2-{5-[AMINO(IMINIO)METHYL]-1H-BENZIMIDAZOL-2-YL}-4-(TRIFLUOROMETHOXY)BENZENOLATE 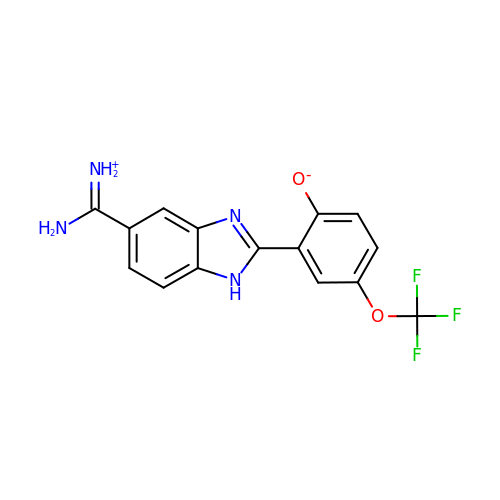| C15 H11 F3 N4 O2 | PJUALJXOBAXGBO-UHFFFAOYSA-N3-oxo-3-{4-[3-(thiophen-2-yl)-1,2,4-oxadiazol-5-yl]piperidin-1-yl}propanenitrile 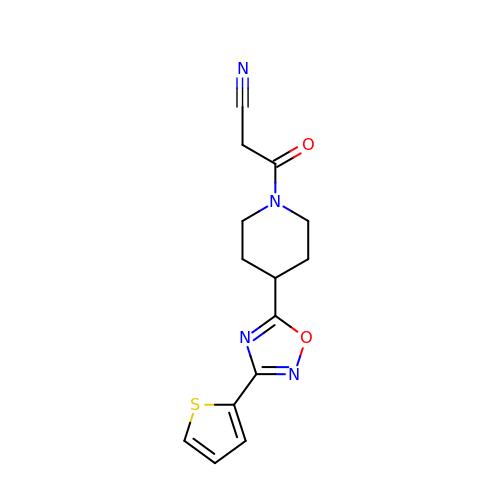| C14 H14 N4 O2 S | SSTGJZVDCOEUFG-UHFFFAOYSA-N> MAHHHHHHMPNRGVVLLDGQALAYSIEKDLKNKIQIITVQVHKRPKLAVILVGKDPASITYVNMKIKACERVGMDFDLKTLQENVTEAELLSLIKDYNTDQNISGVLVQLPLPRHIDSKMVLEAIDPSKDVDGFHPLNIGKLCTQKESFLPATPMGVMRLLKHYHIEIKGKDVAIIGASNIIGKPLSMLMLNAGASVSVCHILTKDISFYTQNADIVCVGVGKPDLIKASMLKKGAV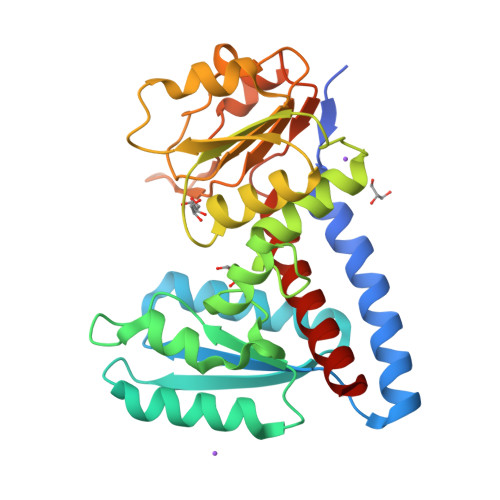VVDIGINHLNDGRIVGDVDFTNAQKVAGFITPVPKGVGPMTIVSLLENTLIAFEKQQRKGF> MENTENSVDSKSIKNLEPKIIHGSESMDSGISLDNSYKMDYPEMGLCIIINNKNFHKSTGMTSRSGTDVDAANLRETFRNLKYEVRNKNDLTREEIVELMRDVSKEDHSKRSSFVCVLLSHGEEGIIFGTNGPVDLKKITNFFRGDRCRSLTGKPK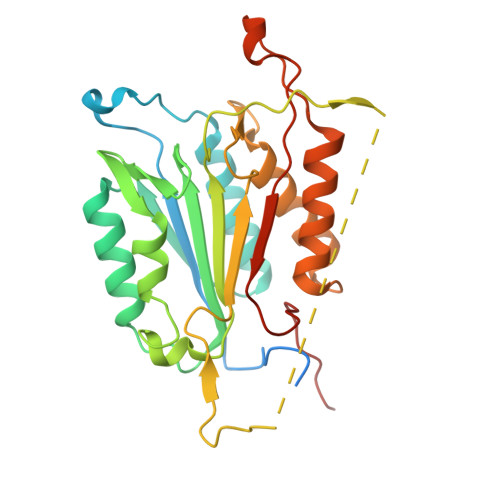LFIIQACRGTELDCGIETDSGVDDDMACHKIPVEADFLYAYSTAPGYYSWRNSKDGSWFIQSLCAMLKQYADKLEFMHILTRVNRKVATEFESFSFDATFHAKKQIPCIVSMLTKELYFYHQLHHHHHH>[2x]GPKGLVPGLVNLGNTCFMNSLLQGLSACPAFIRWLEEFTSQYSRDQKEPPSHQYLSLTLLHLLKALSCQEVTDDEVLDASCLLDVLRMYRWQISSFEEQDAHELFHVITSSLEDERDGSGSHWKSQHPFGVEFETTMKCTESEEEEVTKGKENQDSLSLSIPAATWGHPLTLDHCLHHFISQEEITKQSPTLQRNALYIKSSKISRLPQCLCIHLQRLSWSSHGTPLKRHEHVQFNEDLRLPLAGGRGQA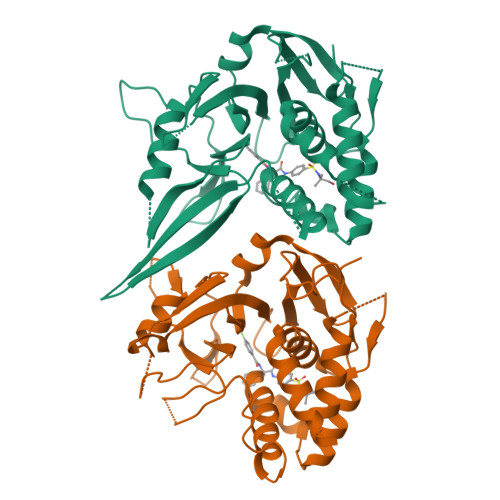YRLMAVVVHHGDMHSGHFVTYRRSPPSARNPLSTSNQWLWVSDDTVRKASLQEVLSSSAYLLFYERV> EFVIEKSLNRIKKFWKEAQYEVIEHSSGLKLVREWDVLEQACKEDLEELVSMKASNYYKIFEQDCLDLESKLTKLSEIQVNWVEVQFYWLDLYGILGENLDIQNFLPLETSKFKSLTSEYKMITTRAFQLDTTIEVIHIPNFDTTLKLTIDSLKMIKSSLSTFLERQRRQFPRFYFLGNDDLLKIIGSGKHHDQVSKFMKKMFGSIESIIFFEDFITGVRSVEGEVLNLNEKIELKDSIQAQEWLNILDTEIKLSVFTQFRDCLGQLKDGTDIEVVVSKYIFQAILLSAQVMWTELVEKCLQTNEFSKYWKEVDMKIKGLLDKLNKSSDNVKKKIEALLVEYLHFNNVIGQLKNCSTKEEARLLWAKVQKFYQKNDTLDDLNSVFISQSGYLLQYKFEYIGIPERLIYTPLLLIGFATLTDSLHQKYGGCFFGPAGTGKTETVKAFGQNLGRVVVVFNCDDSFDYQVLSRLLVGITQIGAWGCFDEFNRLDEKVLSAVSANIQQIQNGLQVGKSHITLLEEETPLSPHTAVFITLNPGYNGRSELPENLKKSFREFSMKSPQSGTIAEMILQIMGFEDSKSLASKIVHFLELLSSKCSSMNHYHFGLRTLKGVLRNCSPLISEFGEGEKTVVESLKRVILPSLGDTDELVFKDELSKIFDSAGTPLNSKAIVQCLKDAGQRSGFSMSEEFLKKCMQFYYMQKTQQALILVGKAGCGKTATWKTVIDAMAIFDGHANVVYVIDTKVLTKESLYGSMLKATLEWRDGLFTSILRRVNDDITGTFKNSRIWVVFDSDLDPEYVEAMNSVLDDNKILTLPNGERLPIPPNFRILFETDNLDHTTPATITRCGLLWFSTDVCSISSKIDHLLNKSYEALDNKLSMFELDKLKDLISDSFDMASLTNIFTCSNDLVHILGVRTFNKLETAVQLAVHLISSYRQWFQNLDDKSLKDVITLLIKRSLLYALAGDSTGESQRAFIQTINTYFGHDSQELSDYSTIVIANDKLSFSSFCSEIPSVSLEAHEVMRPDIVIPTIDTIKHEKIFYDLLNSKRGIILCGPPGSGKTMIMNNALRNSSLYDVVGINFSKDTTTEHILSALHRHTNYVTTSKGLTLLPKSDIKNLVLFCDEINLPKLDKYGSQNVVLFLRQLMEKQGFWKTPENKWVTIERIHIVGACNPPTDPGRIPMSERFTRHAAILYLGYPSGKSLSQIYEIYYKAIFKLVPEFRSYTEPFARASVHLYNECKARYSTGLQSHYLFSPRELTRLVRGVYTAINTGPRQTLRSLIRLWAYEAWRIFADRLVGVKEKNSFEQLLYETVDKYLPNQDLGNISSTSLLFSGLLSLDFKEVNKTDLVNFIEERFKTFCDEELEVPMVIHESMVDHILRIDRALKQVQGHMMLIGASRTGKTILTRFVAWLNGLKIVQPKIHRHSNLSDFDMILKKAISDCSLKESRTCLIIDESNILETAFLERMNTLLANADIPDLFQGEEYDKLLNNLRNKTRSLGLLLDTEQELYDWFVGEIAKNLHVVFTICDPTNNKSSAMISSPALFNRCIINWMGDWDTKTMSQVANNMVDVVPMEFTDFIVPEVNKELVFTEPIQTIRDAVVNILIHFDRNFYQKMKVGVNPRSPGYFIDGLRALVKLVTAKYQDLQENQRFVNVGLEKLNESVLKVNELNKTLPKAPPEEKEASISLVKSLTFEKERWLNTTKQFSKTSQELIGNCIISSIYETYFGHLNERERGDMLVILKRLLGKFAVKYDVNYRFIDYLVTLDEKMKWLECGLDKNDYFLENMSIVMNSQDAVPFLLDPSSHMITVISNYYGNKTVLLSFLEEGFVKRLENAVRFGSVVIIQDGEFFDPIISRLISREFNHAGNRVTVEIGDHEVDVSGDFKLFIHSCDPSGDIPIFLRSRVRLVHFVTNKESIETRIFDITLTEENAEMQRKREDLIKLNTEYRLKLKNLEKRLLEELNNSQGNMLENDELMVTLNNLKKEAMNIEKKLSESEEFFPQFDNLVEEYSIIGKHSVKIFSMLEKFGQFHWFYGISIGQFLSCFKRVFIKKSRETRAARTRVDEILWLLYQEVYCQFSTALDKKFKMIMAMTMFCLYKFDIE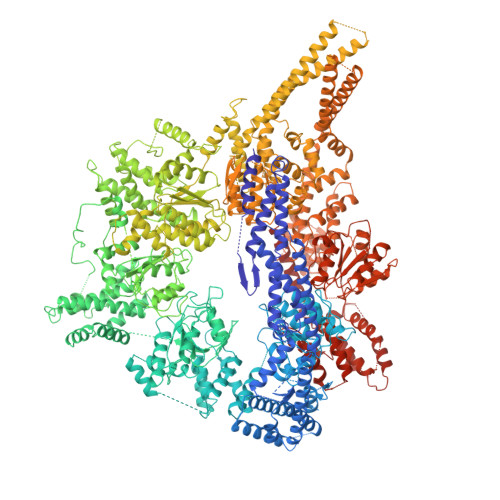SEQYKEAVLTMIGVLSESSDGVPKLTVDTNDDLRYLWDYVTTKSYISALNWFKNEFFVDEWNIADVVANSENNYFTMASERDVDGTFKLIELAKASKESLKIIPLGSIENLNYAQEEISKSKIEGGWILLQNIQMSLSWVKTYLHKHVEETKAAEEHEKFKMFMTCHLTGDKLPAPLLQRTDRVVYEDIPGILDTVKDLWGSQFFTGKISGVWSVYCTFLLSWFHALITARTRLVPHGFSKKYYFNDCDFQFASVYLENVLATNSTNNIPWAQVRDHIATIVYGGKIDEEKDLEVVAKLCAHVFCGSDNLQIVPGVRIPQPLLQQSEEEERARLTAILSNTIEPADSLSSWLQLPRESILDYERLQAKEVASSTEQLLQEM> QDLTVKMTDLQTGKPVGTIELSQNKYGVVFIPELADLTPGMHGFHIHQNGSCASSEKDGKVVLGGAAGGHYDPEHTNKHGFPYTDDNHKGDLPALFVSANGLATNPVLAPRLTLKELKGHAIMIHAG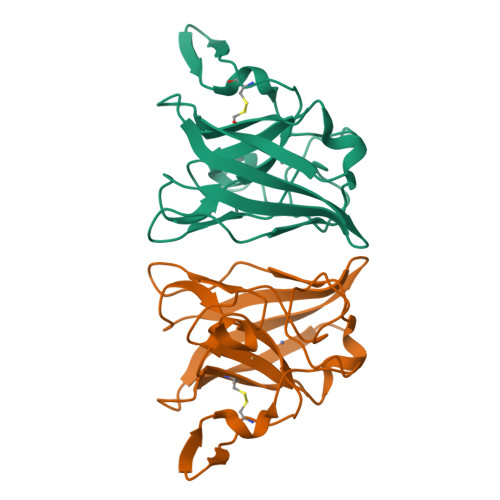GDNHSDMPKALGGGGARVACGVIQ> MPFVNKQFNYKDPVNGVDIAYIKIPNAGQMQPVKAFKIHNKIWVIPERDTFTNPEEGDLNPPPEAKQVPVSYYDSTYLSTDNEKDNYLKGVTKLFERIYSTDLGRMLLTSIVRGIPFWGGSTIDTELKVIDTNCINVIQPDGSYRSEELNLVIIGPSADIIQFECKSFGHEVLNLTRNGYGSTQYIRFSPDFTFGFEESLEVDTNPLLGAGKFATDPAVTLAHELIHAGHRLYGIAINPNRVFKVNTNAYYEMSGLEVSFEELRTFGGHDAKFIDSLQENEFRLYYYNKFKDIASTLNKAKSIVGTTASLQYMKNVFKEKYLLSEDTSGKFSVDKLKFDKLYKMLTEIYTEDNFVKFFKVLNRKTYLNFDKAVFKINIVPKVNYTIYDGFNLRNTNLAANFNGQNTEINNMNFTKLKNFTPLVPR;> RRFAAMLA

The holotoxin is composed of a 100 kDa heavy chain (HC) subunit and a 50 kDa light chain (LC) subunit; these two components are tethered by a disulfide bridge. The LC (BoNT/LC) is a zinc (Zn)(II) metalloprotease that is released from the holotoxin into the neuronal cytosol. Once inside the neuronal cytosol, the LC cleaves specific peptide bonds (depending on the serotype) of proteins composing the neuronal SNARE complex: the synaptosomal-associated protein of 25 kDa (SNAP-25), the vesicle-associated membrane protein (VAMP), also referred to as synaptobrevin, and syntaxin. Of the seven BoNT serotype LCs, the BoNT serotype A LC (BoNT/A LC) possesses the longest duration of action in the neuronal cytosol.

One of the PLMs, JTH-NB72-39, was co-crystallized in complex with the BoNT/A LC protease, confirming the interactions aimed by our design strategy while revealing new, unforeseen inhibitor:enzyme contacts that will preface future studies to design more potent PLM and SMNPI inhibitors. We obtained a co-crystal structure of this complex at 2.4 Å resolution. Significant electron density for the PLM emerged next to the catalytic Zn(II) around the binding cleft defined by loops 70, 250 and 370 in the LC protease. The carbonyl oxygen of the JTH-NB72-39 P1 residue (Arg) coordinates the enzyme's catalytic Zn(II) ion (distance is 2.4 Å) and also engages in a hydrogen bond with the hydroxyl group of residue Tyr 366 (which is known to directly stabilize the tetrahedral intermediate formed during SNAP-25 catalysis), while the amino terminal group of the P1 Arg also coordinates the enzyme's catalytic Zn(II). Specifically, and in contrast to I1, the P1 Arg of the inhibitor engages, via a salt bridge, with the LC's Glu 164 residue while it also shares a hydrogen bond with the carbonyl oxygen of the LC's Cys 165 residue. The amide nitrogen of the JTH-NB72-39 P2′ Phe residue engages in a water mediated interaction with the guanidinium group of BoNT/A LC residue Arg 363. In the present co-crystal structure, Aib engages in favorable intermolecular contacts (via its hydrophobic gem-dimethyl groups) with the side-chain of BoNT/A LC residue Val 70, and an intramolecular, stabilizing, hydrogen bond with the amide nitrogen of its P6′ Leu (not shown). However, the backbone of JTH-NB72-39 abruptly contracts forming a sharp bend at the P3′ position which results from the distinct conformational effects of the Aib residue. The higher Ki value for JTH-NB72-39 compared to I1 is, in part, due to fewer favorable hydrophobic contacts provided by the PLM's Phe component in the P2′ position versus the larger P2′ Trp of I1.> AGSNGAQEKKYIVGFKQTMSTMSAAKKKDVISEKGGKVQKQFKYVDAASATLNEKAVKELKKDPSVAYVEEDHVAHAY;> AQSVPYGVSQIKAPALHSQGYTGSNVKVAVINSGIDSSHPDLNVAGGASFVPSETN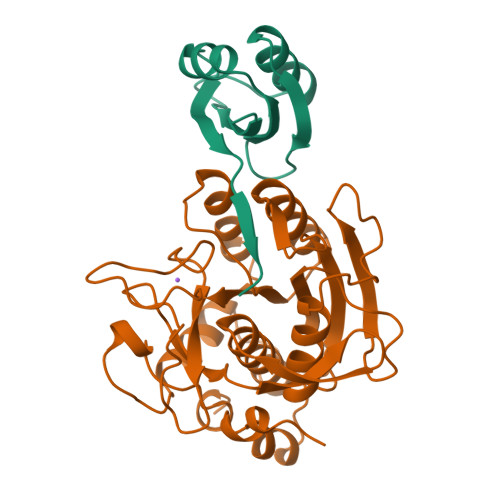PFQDNNSHGTHVAGTVLAVAPSASLYAVKVLGADGSGQYSWIINGIEWAIANNMDVINMSLGGPSGSAALKAAVDKAVASGVVVVAAAGNEGTSGSSSTVGYPGKYPSVIAVGAVDSSNQRASFSSVGPELDVMAPGVSIVSTLPGNKYGAKSGTAMASPHVAGAAALILSKHPNWTNTQVRSSLENTTTKLGDSFYYGKGLINVQAAAQ> GGTGGGGCGCGCCCCACC

Nine new crystal structures of CG-rich DNA 18-mers with the sequence 5′-GGTGGGGGC-XZ-GCCCCACC-3′, which are related to the bacterial repetitive extragenic palindromes, are reported. All 18-mers crystallized as isomorphic tetragonal crystals with one strand of a right-handed antiparallel duplex in the asymmetric unit. All reported structures co-crystallized with the Sr2+ cation located between nucleotides 6 and 7 and (by symmetry) 12 and 13.

All four Chom-18-mers with two central nucleotides (residues 9 and 10) able to form Watson–Crick pairs were crystallized. The topology of the G–C pair is compatible with the Watson–Crick pair, but it was not classified as a pair because its atoms do not comply with the hydrogen-bond geometry. NtC classes provided valuable help with building the initial models of six of the nine 18-mers, i.e. Chom-18-AT, Chom-18-CG, Chom-18-GC, Chom-18-GT, Chom-18-TC and Chom-18-AG. Only Chom-18-CG, Chom-18-GC and Chom-18-AC have all dinucleotides assigned (classified as NtC classes AA##); unassigned dinucleotides (NtC class NANT) are mostly localized near the central base pair.1-({1-[2-({3,5-dimethyl-4-[2-(pyrrolidin-1-yl)ethoxy]phenyl}amino)pyrimidin-4-yl]-4-methyl-1H-pyrrol-3-yl}methyl)azetidin-3-ol 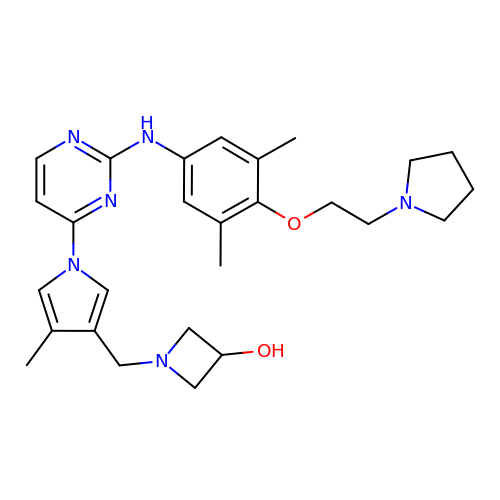| C27 H36 N6 O2 | CXYOUSONGUCKEF-UHFFFAOYSA-N> MDHLKHLQQLQNIERIVLSGIVLANHKIEEVHSVLEPSDFYYPPNGLF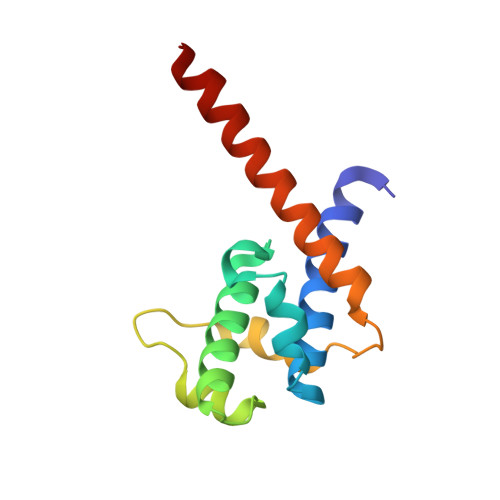FEIALKLHEEDCPIDENFIRQKMPKDKQIKEEDLVAIFAASPIDNIEAYVEEIKNASIKRKLFGLANTIREQAHH> IVGGYTCAANSIPYQVSLNSGSHFCGGSLINSQWVVSAAHCYKSRIQVRLGEHNIDVLEGNEQFINAAKIITHPNFNGNTLDNDIMLIKLSSPATLNSRVATVSLPRSCAAAGTECLISGWGNTK;> SSGSSYPSLLQCLKAP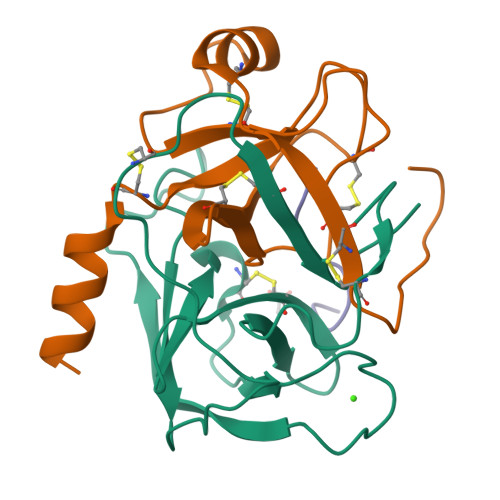VLSDSSCKSSYPGQITGNMICVGFLEGGKDSCQGDSGGPVVCNGQLQGIVSWGYGCAQKNKPGVYTKVCNYVNWIQQTIAAN;> GKDSCQGDS> AQSVPWGISRVQAPAAHNRGLTGSGVKVAVLDTGISTHPDLNIRGGASFVPGEPSTQDGNGHGTHVAGTIAALNNSIGVLGVAPSAELYAVKVLGASGSGSVSSIAQGLEWAGNNGMHVANLSLGSPSPSATLEQAVNSATSRGVLVVAASGNSGAGSISYPARYANAMAVGATDQNNNRASFSQYGAGLDIVAPGVNVQSTYPGSTYASLNGTSMATPHVAGAAALVKQKNPSWSNVQIRNHLKNTATSLGSTNLYGSGLVNAEAATR

The 269 amino acid subtilisin from Bacillus lentus (Savinase) and the homologous subtilisins from B. alcalophilus, B. amyloliquefaciens and B. subtilis are the most studied proteins from this class. The subtilisins comprise a structural family with an α/ β fold and a monomeric nearly spherical structure. The catalytic Asp/Ser/His triad is located in a groove on the surface of the protein. In the structure of Savinase, two structural metal binding sites are found to be occupied by Na+ and Ca2+.

The crystals for both room temperature (RT) and cryogenic datasets were picked from condition G2 of the PACT screen, 0.2 M NaBr, 0.1 M Bis Tris propane pH 7.5, 20% PEG3350. The ambient temperature (RT data) were collected at 297 K, and showed negligible radiation damage; the cryogenic data (cryo data) were collected at 100 K. Images were integrated using XDS and scaled with Aimless. Savinase was crystalized in space group P212121 and diffraction data were collected to 1.1 Å and 0.95 Å resolution for the RT and cryogenic crystals, respectively. qFit and Ringer were used to construct multi-conformer models of Savinase for both the RT and cryogenic crystals. The structures derived from the crystals at room and cryogenic temperatures are very similar, with an RMSD between the structures of 0.20 Å and 0.37 Å for the backbone and all heavy atoms, respectively. Thus, the two structures show no regions with major differences. From the multi-conformer refinement, we find alternative conformations for 28 residues in the RT structure and for 25 residues in the cryo structure. Most of the residues with alternative rotamers are serines, 14/28 and 12/25 in the RT and cryo structures, respectively. Except for the peptide segment 128-132 in the cryo structure and the dipeptide 103-104 in both structures, the residues with alternative conformations are isolated in the structure and do not appear to engage in any cooperative network of conformational change. We have demonstrated that Savinase, except for alternative rotameric states of 25 sidechains is well described by a single conformation for the RT structure. The qFit and Ringer analysis of the crystallographic data did not identify significant minor conformations in this rather rigid enzyme structure.> SGGDGR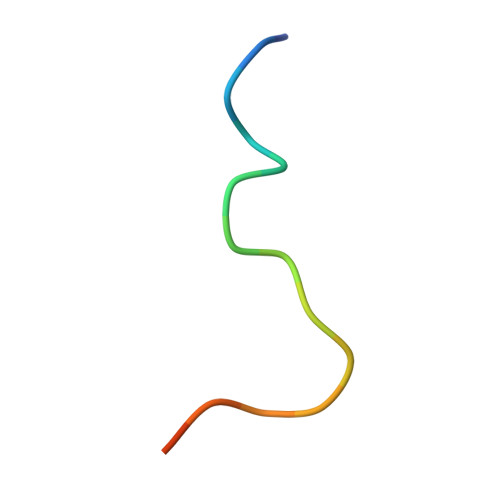GHNTGAHSTSG(S)-CYCLOHEXANONE-2-ACETATE | C8 H12 O3 | 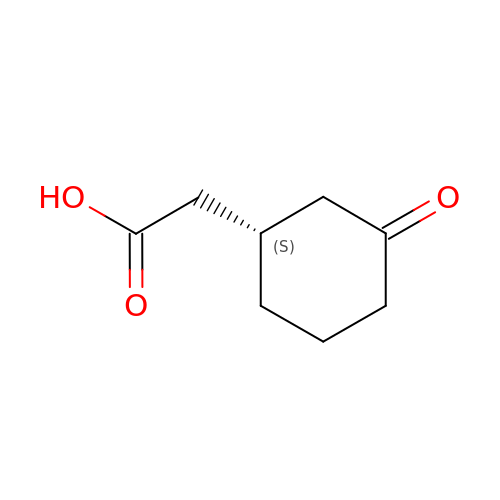RYTWPAUCABOYJP-LURJTMIESA-N>MSKEVSEEAQAHQHGKDYVDPPPAPFFDLGELKLWSFWRAAIAEFIATLLFLYITVATVIGHSKETVVCGSVGLLGIAWAF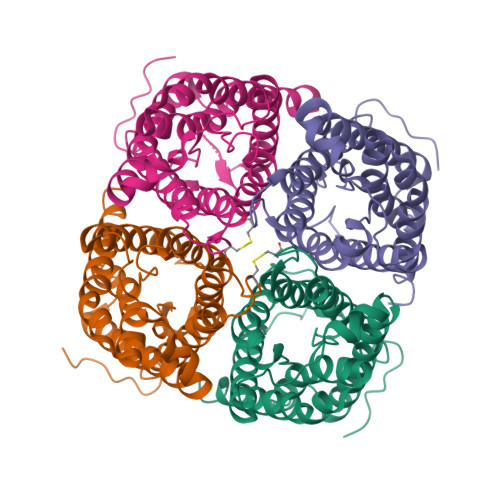GGMIFVLVYCTAGISGGHINPAVTFGLFLARKVSLLRALVYMIAQCLGAICGVGLVKAFMKGPYNQFGGGANSVALGYNKGTALGAEIIGTFVLVYTVFSATDPKRSARDSHVPILAPLPIGFAVFMVHLATIPITGTGINPARSFGAAVIFNSNKVWDDQWIFWVGPFIGAAVAAAYHQYVLRAAAIKALGSFRSNPTNLEQKLISEEDLNSAVDHHHHHH[4x]> SNAMTKKKVYIVSHSHWDREWYLPYEEHHMRLIELVDNVLDLIENDPEFNSFHLDGQTIILDDYLQVRPEKKEAVKKAVQAGKLKIGPFYILQDDFLISSESNVRNMLIGHLESQKWGAPVQLGYFPDTFGNMGQTPQMMQLANLPAAAFGRGVKPIGFDNQVLESDYSSQYSEMWWEGPDQTKIFGLLFANWYSNGNEIPSEKEAAIAFWKQKLADVERYASTNHLLMMNGVDHQPVQRDITKAIALANELFPEYEFIHSNFDDYLKAVQEELPEDLGTVTGELTSQETDGWYTLANTSSARVYLKQWNTKVQRQLENIAEPLAAMAYEVTGDYPHDQFDYAWKTLLQNHPHDSICGCSVDEVHRGMMTRFENANDVGHFLADEATRQLTEAIDTSVFPEKAHPFVLFNTSGYQKTEVVTVEVEIERLPFYTGKPEDLYHELKQKATPDYQVIDPTGKAVASRIVKEDVRFGYDLPKDAFRQPYMAKYLTVELSVKEMAPFSWDSFALIQGETKAFEGSLLAQPATNEME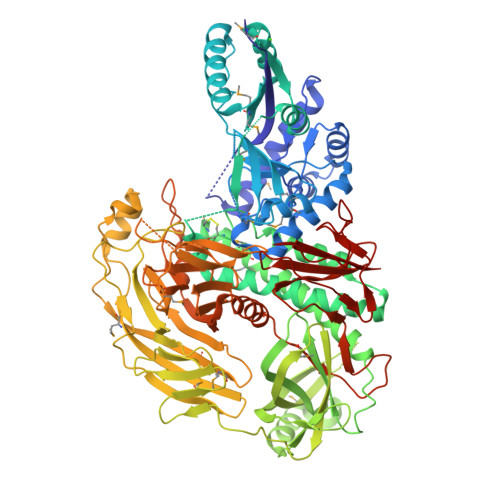NEFIQVKIENNGSLTIADKKTGETFSKLLTFEDTGDIGNEYIFFKPTEDQGITTENVTAEITNKENSPVKASYQIKQTVMLPVAADERLEEEQKAVREFRERLAQRSTTLRPFEITTMVTMIKESNQLFFETTINNQIKDHRLRVLFPTGMVTETHEADSIYEVVTRPNQVSDTWENPTNPQHQQAFVNVHDQNKGVTIFNEGLNEYEVLADGTIAVTLIRCVGELGDWGYFATPEAQCQGEYTFKYGLSLHGKPEERFATYQQAYSAQIPFTAATTARHEGKLAPNHVYLTTAEGPIGWTAVKRQEQTNHLVVRGFNLTAQNIPCELHKETQPATCLTNVLEEPLTPAIEVDAPLRPFEIRTWRFEK> SKVALITGVTGQDGSYLAEFLLEKGYEVHGIKRRASSFNTERVDHIYQDPHTCNPKFHLHYGDLSDTSNLTRILREVQPDEVYNLGAMSHVAVSFESPEYTADVDAMGTLRLLEAIRFLGLEKKTRFYQASTSELYGLVQEIPQKETTPFYPRSPYAVAKLYAYWITV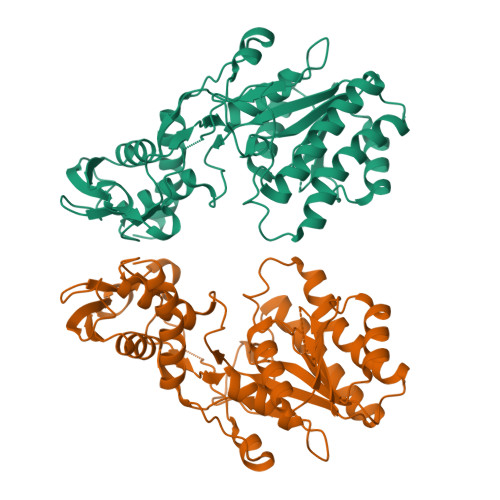NYRESYGMYACNGILFNHESPRRGETFVTRKITRAIANIAQGLESCLYLGNMDSLRDWGHAKDYVKMQWMMLQQEQPEDFVIATGVQYSVRQFVEMAAAQLGIKLRFEGTGVEEKGIVVSVTGHDAPGVKPGDVIIAVDPRYFRPAEVETLLGDPTKAHEKLGWKPEITLREMVSEMVANDLEAAKKHSLLKSHGYDVAIALES O-linked β-N-acetyl-D-glucosamine (O-GlcNAc) transferase (OGT) and hydrolase (OGA) control a dynamic, reversible, and tightly regulated post-translational modification termed O-GlcNAcylation. OGT possesses 13.5 tetratricopeptide repeats (TPRs) at the N terminus, which harbor all currently known ID-associated mutations (Lubas et al., 1997). In OGT, the TPRs form a 120-Å superhelix, which serves as a potential interaction surface for substrates and binding partners (Jínek et al., 2004, Zeytuni and Zarivach, 2012). Recently, mutations in the N terminus of human OGT have been associated with ID, namely, A319T, L254F, R284P, and Δ155-177 (Bouazzi et al., 2015, Niranjan et al., 2015, Willems et al., 2017).

The ID-associated mutation L254F (Vaidyanathan et al., 2017) is located on TPR helix 7, distant from the active site. To investigate structural changes attributable to the L254F mutation, we determined the crystal structure of the mutant TPR domain (TPRL254F). Diffraction data were collected to 1.75 Å and initial refinement starting from the TPRWT structure required substantial rebuilding of the terminal TPRs, an early indication of considerable conformational changes. In wild-type OGT, L254 occupies the interface between the helices of TPR7, with its side chain constricted in a pocket formed by the surrounding residues N223, L225, Y228, and R250. Mutation of L254 to the bulkier Phe appears to be accommodated in this pocket, however, by causing small changes in torsion angles of the residues lining the pocket and by displacing TPR helix 7B away from helix 7A by 1.5 Å. Increasing shifts of the TPRs starting from the mutation site lead to a maximum shift of 12 Å for the N-terminal TPR. The melting curve for TPRL254F was shifted, yielding a Tm of 55°C, indicative of reduced thermal stability. In sTPRL254F conformation 1 (sTPRL254F-C1), the F254 side chain occupies the same position as observed in the TPRL254F crystal structure, while in sTPRL254F conformation 2 (sTPRL254F-C2), the F254 phenyl moiety interacts with the side chains of N223, L225, and Y228 and the backbone of the F224 and R250. Thus, the L254F mutation destabilizes the interface between TPRs 6 and 7. The data presented here show that the L254F mutation causes a subtle structural distortion at the mutation site that propagates through the TPR superhelix, resulting in a substantial displacement of the N-terminal TPRs and a markedly increased structural plasticity compared with the TPRWT.

> GPMELAHREYQAGDFEAAERHCMQLWRQEPDNTGVLLLLSSIHFQCRRLDRSAHFSTLAIKQNPLLAEAYSNLGNVYKERGQLQEAIEHYRHALRLKPDFIDGYINLAAALVAAGDMEGAVQAYVSALQYNPDLYCVRSDLGNLLKALGRLEEAKACYLKAIETQPNFAVAWSNLGCVFNAQGEIWLAIHHFEKAVTLDPNFLDAYINLGNVLKEARIFDRAVAAYLRALSFSPNHAVVHGNLACVYYEQGLIDLAIDTYRRAIELQPHFPDAYCNLANALKEKGSVAEAEDCYNTALRLCPTHADSLNNLANIKREQGNIEEAVRLYRKALEVFPEFAAAHSNLASVLQQQGKLQEALMHYKEAIRISPTFADAYSNMGNTLKEMQD Histone deacetylase (HDAC) enzymes catalyze the deacetylation of histone and non-histone proteins. Out of the family of 11 HDAC isozymes, HDAC6 has emerged as a highly attractive and safe target in drug discovery, because of its imperative roles in cellular function and survival, and well-tolerated loss of function when inhibited. The cytoplasmic clients of HDAC6 include an extensive substrate repertoire such as α-tubulin, cortactin, HSP90, tau and peroxiredoxins. HDAC inhibitors typically consist of a cap group which interacts with the surface of the enzyme, a zinc binding group (ZBG) that interacts with the zinc ion in the catalytic pocket, and a linker between these two moieties.

The X-ray crystal structure of the HDAC6–NN-390 complex, which was solved at 1.6 Å resolution, displays a similar profile of contacts in the catalytic tunnel when compared to that of HDAC6-ricolinostat complex. Unlike that of the HDAC6-TO-317 complex, the hydroxamate moiety coordinates to the catalytic Zn2+ ion in a bidentate fashion. The hydroxamate N-O group coordinates to Zn2+ with an average separation of 2.2 Å and the hydroxamate C=O group with a distance of 2.34 Å. Alongside these contacts, interaction of NN-390 completes the canonical 5-membered chelate complex via a hydrogen bond network. The chelate complex involves the side chains Y745 (O—O distance = 2.44 Å), H574 (N—N distance = 2.62 Å), and H573 (N—O distance = 2.47 Å), the latter of which is unobserved for TO-317. The hydroxamate moiety of NN-390 is further able to engage in hydrophobic interactions with D612, D705, and H614, similar to that of ricolinostat. The H614 side chain makes Van der Waals contacts with the benzyl group of the phenylhydroxamate moiety and the isopropyl side group in NN-390, the latter of which is mediated via a water molecule. The benzyl group is sandwiched between F583 and F643 and establishes π-π stacking interactions. The F583 side chain alongside L712 chain also engages in Van der Waals contacts with one of the oxygen atoms of the sulfonamide moiety. Although relatively weakly resolved, and likely more dynamic, the tetra-fluorobenzene (TFB) capping group is observed to make weak interactions with the side chain of H463 and that of S531 and F583 via distinct water molecules.

> PITGLVYDQRMMLHHNMWDSHHPELPQRISRIFSRHEELRLLSRCHRIPARLATEEELALCHSSKHISIIKSSEHMKPRDLNRLGDEYNSIFISNESYTCALLAAGSCFNSAQAILTGQVRNAVAIVRPPGHHAEKDTACGFCFFNTAALTARYAQSITRESLRVLIVDWDVHHGNGTQHIFEEDDSVLYISLHRYEDGAFFPNSEDANYDKVGLGKGRGYNVNIPWNGGKMGDPEYMAAFHHLVMPIAREFAPELVLVSAGFDAARGDPLGGFQVTPEGYAHLTHQLMSLAAGRVLIILEGGYNLTSISESMSMCTSMLLGDSPPSLDHLTPLKTSATVSINNVLRAHAPFWSSLR> MSQNNTISSMNPERAYNNVTLKNLTAFQLLSQRENICELLNLVESTERHNSIINPERQRMSLEEMKKMLDALKNERKK;> MSGSNMGYYDVLAGLSALEKSSQVVFSATELQQLTQQSHATDKGIEGSENSKAKVSKPKRVAVHGYLGGKVSLADAAQVEYEVGHSLLGSYVPRQQLEALSSVDFSHHFHRTLECKAALETHDVFLAGAGQLSLPFQSHIESPRNSEAKRKRKVIICKRCQSRFIGSHRRSQLREHACVD;> MSDSEGGLASEVEHEKRSRSTSNRPNYAIDTEDLDIDENDENEDDDYREEEANEGVNEEEISDEEEQINKSGRNKRRHVDEEEDLSEDKGVTRSRNRSKFKKPVFPGIDDAEENLNPLKVVNEEYVLPDDPEGETKITADGDLLGGREFLVRTFTLTEKGNRKFMLATEPARIVGFRDSYLFFQTHPNLYKFILNQTQKNDLIDRGVLPYSYRNRQIALVTARGVFKEFGAKIIRGGKHITDDYYASELRTKGNVIEGKLAGDPIDKSARALETMMYPASENGINPAKNQVEFFEHRPHGHMSNSNIIASGSKLSSTNWLYQHSAACSRFNSDLFYDRVKVLLVDQQGLRDAYTNILHIPESTQSTTVLGWRRSKNDSPSDTSIVYETVIHDNDLNKPKTGLSEIPKEIYEDVVDEDVLRAITEQQNFEKCNEYI;> MMPDDNSNSSTQNSSALYKDLRKEYESLFTLKEDSGLEISPIFNVLPPKKDYPDYYAVIKNPVSFNTLKKRIPHYTDAQQFMNDVVQIPWNAKTYNTRDSGIYKYALVLEKYLKDTIYPNLKEKYPQLVYPDLGPLPDEPGYEEFQQKLREKAEEVARANAARAESSSSMNSTEAARRLRKTRTSVKRESEPGTDTNNDEDYEATDMDIDNPKDADFPDLIRKPLININPYTRKPLRDNRSTTPSHSGTPQPLGPRHRQVSRTQVKRGRPPIIDLPYIQRMKNVMKVLKKEVLDSGIGLTDLFERLPDRHRDANYYIMIANPISLQDINKKVKTRRYKTFQEFQNDFNLMLTNFRISHRGDPESIKISNILEKTFTSLARFELSKPDRSFIPEGELRYPLDEVIVNNISYHVGDWALLRNQNDPQKPIVGQIFRLWKTPDGKQWLNACWYYRPEQTVHRVDRLFYKNEVMKTGQYRDHLVSNLVGKCYVIHFTRYQRGNPDMKLEGPLFVCEFRYNESDKIFNKIRTWKACLPEEIRDLDEATIPVNGRKFFKYPSPIRHLLPANATPHDRVPEPTMGSPDAPPLVGAVYMRPKMQRDDLGEYATSDDCPRYIIRPNDSPEEGQVDIETGTITTNTPTANALPKTGYSSSKLSSLRYNRSSMSLENQNAIGQQQIPLSRVGSPGAGGPLTVQGLKQHQLQRLQQQQHQYQQQKRSQASRYNIPTIIDDLTSQASRGNLGNIMIDAASSFVLPISITKNVDVLQRTDLHSQTKRSGREEMFPWKKTKGEILWFRGPSVIVNERIINSGDPHLSLPLNRWFTTNKKRKLEYEEVEETMEDVTGKDKDDDGLEPDVENEKESLPGPFVLGLRPSAKFTAHRLSMLRPPSSSS;> MDIRGRKMKKPPACVQCRKRKIGCDRVKPICGNCMKHNKMDCFYPDVPGQYVPSSSSSSNTRQVANGPYLNSYYASRRVSKETAALLQKNPELASLEQIREYNTRLQLLNAQNQLNNRSSAANATLNQQHTQYIPKSVPSLESKPVTSANESSTPLNWVQGPAIFHMLTSPYTQDEIINHEMNFLKGRLLELQEITGKKITGVNLDLKQDSSAQMQSSHSNRNQEEFLTIKKRKLSEDGVTDGDGKPIPESERRPHLNEFKDLDPQFLDTNKVFNVFNSAISEEGRNRLWLLPKNINKSSIFQIQYLIERDPFLFKFFNDLNILIETQFNGPLHDLVASRNSIERNSGISQILKFPSQSITQTLINKYLSTITETNSILPILKPKRLLPIVEQLFPSNTINKPNSKDFETIFQVFSVTNDQLLNLGFITLCLLILFESLNSTVLIPLRDDEHLQLFNVLFNYLPLLKSNLTTLRFEIEKRSMCNIETLRFISLWKYYQFVMDTSSSSSFVIDYDEDMHMACLLSLNHETQNQSHILTWNFIFKNYCWRHLFLGQLPLLMSEPFTNSTPIIDPLLNNDFELIDFEVNLMKYLQSKDQQLSIDKIIQLIKLLKNKNIEVSQGCLTTPSIINNIMDSLIYRNSMLYLNFYLLLQFETLKNYAKFNEILEDFLELSRETLFFVFSNLANIKFAGHEFTFINKSIVVLQTLVLMLLALYQRSFDSSKRTNDANEISEQTDIHSNNDNSKRIKNKNVIHLIINKIAMLLSDYSKNCKKQNKLIENLIIKIKTISKYIKNLEENKVTTSADSNYSINNGFSGISAEQLIKLNHELSKISESLIKTDFYEQRKNSTVSNGVLGAAAPVDSDANSDTFGLTKENFNEVFEAIRS;> MVVKKRKLATEAGGSDERPKYLPGKHPKNQEKTPHVDYNAPLNPKSELFLDDWHIPKFNRFISFTLDVLIDKYKDIFKDFIKLPSRKFHPQYYYKIQQPMSINEIKSRDYEYEDGPSNFLLDVELLTKNCQAYNEYDSLIVKNSMQVVMLIEFEVLKAKNLKRNYLINSEVKAKLLHYLNKLVDATEKKINQALLGASSPKNLDDKVKLSEPFMELVDKDELPEYYEIVHSPMALSIVKQNLEIGQYSKIYDFIIDMLLVFQNAHIFNDPSALIYKDATTLTNYFNYLIQKEFFPELQDLNERGEINLEFDKFEFENYLAIGGGGPAAAGALAISALDNDIEPESNREDLIDQADYDFNHFEGLGNGYNRSLLTEDYLLNPNNFKKLIAKPETVQSEVKNERSTTSDIEKTNSLESEHLKIPKYNVIKSMQKEMQSLSEQHTMEYKPYKLIQQIYIFSSKNLYSQATKPLLGSRPSCNQNWVEYIFNGNELSQNENAFSFMLQPMQTFLTLQSHLTSSLKDTETLLTINKEPVKSRTSNVNSNLSQPQQQENDVIGNDTKQDIENLTIGGGNNNDIVGNDNDKRNNITEIFDIRLSEGLNHLMFRCEDKISHETEFMNFWINVLP;>[4x]MSDTEKDKDVPMVDSHEATEEPPTTSTNTPSFPHLAQEQAKEESATLGAEVAHKKINYEQEAQKLEEKALRFLAKQTHPVIIPSFASWFDISKIHEIEKRSNPDFFNDSSRFKTPKAYKDTRNFIINTYRLSPYEYLTITAVRRNVAMDVASIVKIHAFLEKWGLINYQIDPRTKPSLIGPSFTGHFQVVLDTPQGLKPFLPENVIKQEVEGGDGAEPQVKKEFPVNLTIKKNVYDSAQDFNALQDESRNSRQIHKVYICHTCGNESINVRYHNLRARDTNLCSRCFQEGHFGANFQSSDFIRLENNGNSVKKNWSDQEMLLLLEGIEMYEDQWEKIADHVGGHKRVEDCIEKFLSLPIEDNYIREVVGSTLNGKGGDSRDGSVSGSKLMECVNDAVQTLLQGDDKLGKVSDKSREISEKYIEESQAIIQELVKLTMEKLESKFTKLCDLETQLEMEKLKYVKESEKMLNDRLSLSKQILDLNKSLEELNVSKKLVLISEQVDSGIQLVEKDQEGDDEDGNTATGHGVKRVGKEGEEVGEGDSIAKLQPQVYKPWSL;> MVTQTNPVPVTYPTDAYIPTYLPDDKVSNLADLKKLIEMDSRLDLYLTRRRLDTSINLPTNTKTKDHPPNKEMLRIYVYNTTESSPRSDSGTPADSGKTTWTLRIEGKLLHESANGKHPFSEFLEGVAVDFKRLKPLGMGKKRKRDSSLSLPLNLQQPEYNDQDSTMGDNDNGEDEDSAEAESREEIVDALEWNYDENNVVEFDGIDIKRQGKDNLRCSITIQLRGVDGGKVQYSPNLATLIGMQTGSVNDAVYSIYKYILINNLFVTEQTEAQDGSNDAEDSSNENNNKNGAGDDDGVEGSTPKDKPELGEVKLDSLLQKVLDTNAAHLPLMNVVQTVNKLVSPLPPIILDYTIDLSKDTTYGATTLDVDVSHILHQPQPQPNLQKEEETDAEDTAKLREITKLALQLNSSAQKYQFFHELSLHPRETLTHYLWSSKQNELVLQGDQYFNEDAARTSDIYSNNNNDRSLMGNISLLYSQGRL;> MNSLASNTPLNGTPVSEAPATSSEPVNMFETMVANPIKVSRLQSNGVLTGPAANTKSIHYSLANFNVFQSLPKETARGVDDLTRMEMALLSGIPEEIKWSLKKYLTYSNKAPYMISLRTLPDLLPLFKTFILPLERIVEGLNKSSICDSKAMDSLQMGLNALLILRNLAQDTDSVQILVKDREIKSFILFILKKFQCVATGDNKWQLYEGNATFFNELTHYTLDLMEAISSYIAPAMKDDHYFQTLVSILNYTKDRYMVISILRSLSRLLVRSKANEESAADNLDHKTLSLIVSFLLLECDSELIIASLDFLYQYILPGSQRITELFKSKECSLILEATLPNLLSYNIATPDYHLLQKHKIRLIKRLKPPAPKEPPNLSEDLFQQLFKLNEPLRSTAWLRCCFEPVQEAEFTQISLWRSYESKFGQPVRESGRKLLPAVEFIKNVSNAFNNAAAIVITDPVTGKKRFVIKGIQPRFKALGIADGERESQVPISALKSKFLNDSKEITPARQNSIPEVKFPQELSDVSKVACTFLCLLSNDTDDGAGSAFCQRIRPLVLHKLADIPPLTLALSEYMENTSGL;> MTESVGGNKLVDFLVNVQSILNAASVKCHVVDESFPAKFFEKNPDKIYESYCKFIKNRSNSEGLIRNEDKLVLTTINKRFENGEYEPIQGGFYKLYHDIKLVCTILIHFYPQGTRNYQLVDKFYKFSSELLLRECCRIGIALTQTNNIKSRSGKLLSGNEMDEYDDDDATELDKIISYDFIKISMNYTVPISQTYQIRTKDMDLFSSIISKSNLDKRPHELPNTNFKINNVLPQTDIENEAPRLGFVGANTSNIPDPTLPPTEMMTRFLHPNWYALPTTVWLKYGNYNSWAPSFNENGTVVDSTTRGLIWLERIGYMDLYEKNEKKVKQEELLNTNEEGINRKQNDENNKNVDGKSNGVQDDGGDNDNDATIASANSESTENKEQFIIKLQNLYNWTPSNYIGDDEIENFRNGTPDKLVSDSLLKLKRLRKERILNKVLKPTTEERELYFKVKRILKEVILAKKVSKVPINNVRAFPVLQTNYNGSIPVVRAQPGRKRKHKK;> MSHQNQLIPQAYISNFHNRLTNEDDGIPIFTMAQQTRQHKRAKVVNYAEYDNDLFDEFNMNGSNFNNADTHYKDNAVSHENTPALTNGVTMDGSEYNVLENMNGADSIISNNKYDAGSNMVVESLSGLNSNNNASNGPSNKAQAQDIGNAVLPDLQDQHHNPFNILRYPKIRDTFINGKVVSPYRLNTDQETKANANSGEAIMIPITLDIEHMGHTIKDQFLWNYNDDSISPEEFASIYCKDLDMTSATLQTQIANIIKEQLKDLENIAATEIMSDLHVIINLTCNLQDRFFEDNFQWNLNDKSLTPERFATSIVQDLGLTREFIPLISQSLHETILKIKKDWVDGHLIQDHVPNDAAFGYLSGIRLDIDELGSNWCPRVEILTKEEIQKREIEKERNLRRLKRETDRLSRRGRRRLDDLETTMRM;> MLQEQSELMSTVMNNTPTTVAALAAVAAASETNGKLGSEEQPEITIPKPRSSAQLEQLLYRYRAIQNHPKENKLEIKAIEDTFRNISRDQDIYETKLDTLRKSIDKGFQYDEDLLNKHLVALQLLEKDTDVPDYFLDLPDTKNDNTTAIEVDYSEKKPIKISADFNAKAKSLGLESKFSNATKTALGDPDTEIRISARISNRINELERLPANLGTYSLDDCLEFITKDDLSSRMDTFKIKALVELKSLKLLTKQKSIRQKLINNVASQAHHNIPYLRDSPFTAAAQRSVQIRSKVIVPQTVRLAEELERQQLLEKRKKERNLHLQKINSIIDFIKERQSEQWSRQERCFQFGRLGASLHNQMEKDEQKRIERTAKQRLAALKSNDEEAYLKLLDQTKDTRITQLLRQTNSFLDSLSEAVRAQQNEAKILHGEEVQPITDEEREKTDYYEVAHRIKEKIDKQPSILVGGTLKEYQLRGLEWMVSLYNNHLNGILADEMGLGKTIQSISLITYLYEVKKDIGPFLVIVPLSTITNWTLEFEKWAPSLNTIIYKGTPNQRHSLQHQIRVGNFDVLLTTYEYIIKDKSLLSKHDWAHMIIDEGHRMKNAQSKLSFTISHYYRTRNRLILTGTPLQNNLPELWALLNFVLPKIFNSAKTFEDWFNTPFANTGTQEKLELTEEETLLIIRRLHKVLRPFLLRRLKKEVEKDLPDKVEKVIKCKLSGLQQQLYQQMLKHNALFVGAGTEGATKGGIKGLNNKIMQLRKICNHPFVFDEVEGVVNPSRGNSDLLFRVAGKFELLDRVLPKFKASGHRVLMFFQMTQVMDIMEDFLRMKDLKYMRLDGSTKTEERTEMLNAFNAPDSDYFCFLLSTRAGGLGLNLQTADTVIIFDTDWNPHQDLQAQDRAHRIGQKNEVRILRLITTDSVEEVILERAMQKLDIDGKVIQAGKFDNKSTAEEQEAFLRRLIESETNRDDDDKAELDDDELNDTLARSADEKILFDKIDKERMNQERADAKAQGLRVPPPRLIQLDELPKVFREDIEEHFKKEDSEPLGRIRQKKRVYYDDGLTEEQFLEAVEDDNMSLEDAIKKRREARERRRLRQNGTKENEIETLENTPEASETSLIENNSFTAAVDEETNADKETTASRSKRRSSRKKRTISIVTAEDKENTQEESTSQENGGAKVEEEVKSSSVEIINGSESKKKKPKLTVKIKLNKTTVLENNDGKRAEEKPESKSPAKKTAAKKTKTKSKSLGIFPTVEKLVEEMREQLDEVDSHPRTSIFEKLPSKRDYPDYFKVIEKPMAIDIILKNCKNGTYKTLEEVRQALQTMFENARFYNEEGSWVYVDADKLNEFTDEWFKEHSS;> MMDMQVRKVRKPPACTQCRKRKIGCDRAKPICGNCVKYNKPDCFYPDGPGKMVAVPSASGMSTHGNGQGSNHFSQGNGVNQKNVMIQTQYPIMQTSIEAFNFSFNPSVDTAMQWTKAASYQNNNTNNNTAPRQNSSTVSSNVHGNTIVRSDSPDVPSMDQIREYNTRLQLVNAQSFDYTDNPYSFNVGINQDSAVFDLMTSPFTQEEVLIKEIDFLKNKLLDLQSLQLKSLKEKSNLNADNTTANKINKTGENSKKGKVDGKRAGFDHQTSRTSQSSQKYFTALTITDVQSLVQVKPLKDTPNYLFTKNFIIFRDHYLFKFYNILHDICHINQFKVSPPNNKNHQQYMEVCKVNFPPKAIIIETLNSESLNNLNIEEFLPIFDKTLLLEFVHNSFPNGDTCPSFSTVDLPLSQLTKLGELTVLLLLLNDSMTLFNKQAINNHVSALMNNLRLIRSQITLINLEYYDQETIKFIAITKFYESLYMHDDHKSSLDEDLSCLLSFQIKDFKLFHFLKKMYYSRHSLLGQSSFMVPAAENLSPIPASIDTNDIPLIANDLKLLETQAKLINILQGVPFYLPVNLTKIESLLETLTMGVSNTVDLYFHDNEVRKEWKDTLNFINTIVYTNFFLFVQNESSLSMAVQHSSNNNKTSNSERCAKDLMKIISNMHIFYSITFNFIFPIKSIKSFSSGNNRFHSNGKEFLFANHFIEILQNFIAITFAIFQRCEVILYDEFYKNLSNEEINVQLLLIHDKILEILKKIEIIVSFLRDEMNSNGSFKSIKGFNKVLNLIKYMLRFSKKKQNFARNSDNNNVTDYSQSAKNKNVLLKFPVSELNRIYLKFKEISDFLMEREVVQRSIIIDKDLESDNLGITTANFNDFYDAFYN

SWI/SNF chromatin remodelers reposition nucleosomes by translocating DNA around the histone octamer, and in vitro assays have shown that they move nucleosomes to the ends of linear DNA fragments before evicting the histones from the DNA. RSC has a molecular weight of ~1.1 MDa and is composed of 17 proteins, with two copies of Rsc8 and one copy of either Rsc1 or Rsc2. Seven of the proteins (Arp7, Arp9, Rsc6, Rsc8, Sfh1, Sth1 and Rsc9) are conserved in all eukaryotic SWI/SNF chromatin remodeling complexes, with Sth1 containing the ATPase domain that is responsible for the remodeling activity. We found that RSC is composed of five main lobes, three that form a relatively rigid core (head, body and arm) and two that are flexibly attached (leg and tail).

The core of the complex was resolved to 3 Å, which allowed us the de novo building of this entire region. An asymmetric Rsc8 dimer defines the backbone for the complex, scaffolding the three core lobes and contacting all core proteins except Rsc3 and Rsc30. Rsc8 has four conserved domains, which are, from N to C terminus: SWIRM, ZZ, SANT, and coiled coil (CC). The SWIRM domains are in the arm, the ZZ and SANT domains in the head and the CC domains in the body. The body lobe of RSC contains a helical bundle backbone, an α-solenoid belly and a β-sandwich hook. The helical bundle is made up of the two CC domains of Rsc8, along with the CC domains of Rsc6 and Htl1. This helical bundle interacts with the α-solenoid belly made up of the armadillo repeats of Rsc9 and the SwiB domain of Rsc6. Four proteins contribute to most of the arm lobe, which is made of the two SWIRM domains of Rsc8 held together by the Scaffold domain of Npl6 and the RPT1 and RPT2 domains of Sfh1. Six RSC subunits contribute majorly to the head lobe of RSC, which is made of the ZZ and SANT domains of the two copies of Rsc8, the BrD and Scaffold II domain of Rsc58, the Scaffold I and part of Scaffold II domain of Sth1, the β-barrel domain of Rsc4 and the anchor domain of Rsc1/2.>[4x]MNRWQGIIKQYKKYLPVDENTPIVTLYEGNTPLIEADNLARAIGFKGKIYLKYEGLNPTGSFKDRGMTLAISKAVEAGKRAVICASTGNTSASAAAYAARAGLRAYVLLPKGAVAIGKLSQAMIYGAKVLAIQGTFDDALNIVRKIGENFPVEIVNSVNPYRIEG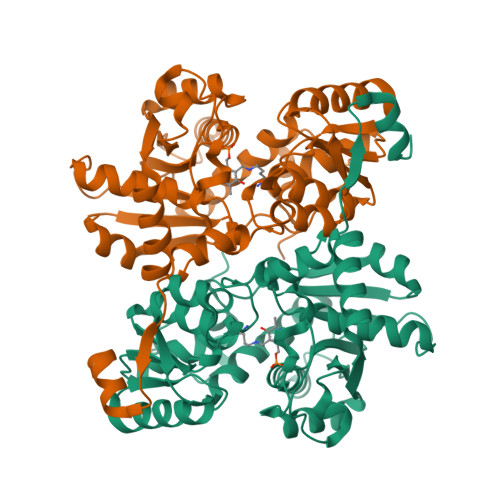QKTAAFEICDTLGEAPDYHFIPVGNAGNITAYWKGFKIYYEEGKITKLPRMMGWQAEGAAPIVKGYPIKNPQTIATAIKIGNPYSWKSALKAAQESGGKIDAVSDSEILYAYKLIASTEGVFCEPASAASVAGLIKLVREGFFKGGEVVTCTLTGNGLKDPDTAIKVCEEPITVPPDFDEVVKVLGF>ALKGSLEGMILERISRGETYGYEITKYLNDL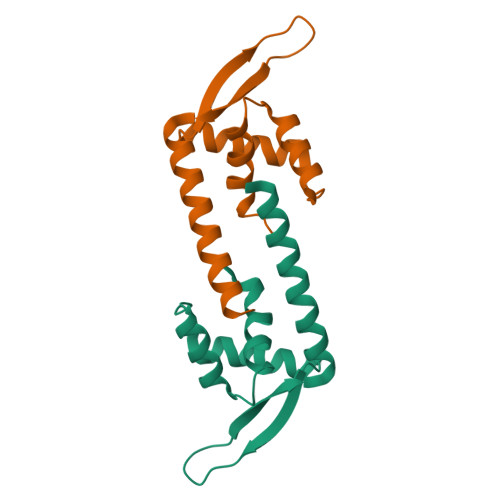GFDEIVEGTVYTILVRLEKKGLVEIEKKKSELGPPRKFYTLSPAGEEELAIFWKRWDFIQGKIMQVK[2x]> EVLTGGHSVSAPQENRIYVMDSVFMHLTESRVHVYDYTNGKFLGMVPTAFNGHVQVSNDGKKIYTMTTYHERITRGKRSDVVEVWDADKLTFEKEISLPPKRVQGLNYDGLFRQTTDGKFIVLQNASPATSIGIVDVAKGDYVEDVTAAAGCWSVIPQPNRPRSFMTICGDGGLLTINLGEDGKVASQSRSKQMFSVKDDPIFIAPALDKDKAHFVSYYGNVYSADFSGDEVKVDGPWSLLNDEDKAKNWVPGGYNLVGLHRASGRMYVFMHPDGKEGTHKFPAAEIWVMDTKTKQRVARIPGRDALSMTIDQQRNLMLTLDGGNVNVYDISQPEPKLLRTIEGAAEASLQVQFHP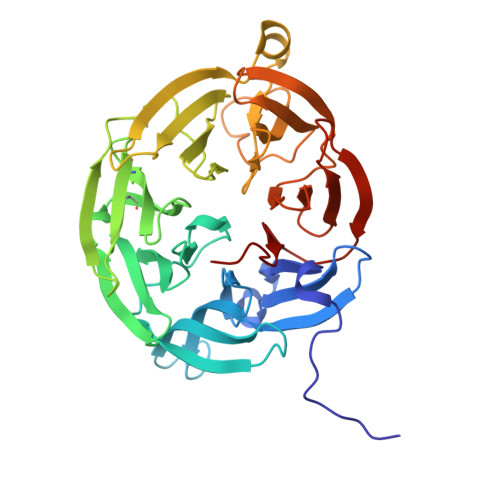VGGT3-[methyl-[2-[methyl-(1-methylpiperidin-4-yl)amino]quinazolin-4-yl]amino]propanenitrile | C19 H26 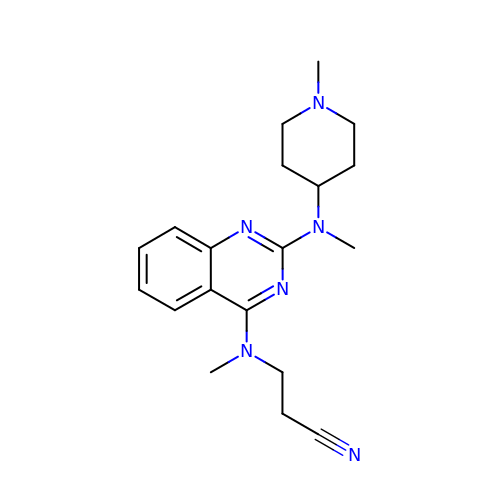N6 | MSXKDQJJTLQTRK-UHFFFAOYSA-N>SMALEIHMSDPMCLIENFNEQLKVNQEALEILSAITQPVVVVAIVGLYRTGKSYLMNKLAGKNKGFSVASTVQSHTKGIWIWCVPHPNWPNHTLVLLDTEGLGDVEKADNKNDIQIFALALLLSSTFVYNTVNKIDQGAIDLLHNVTELTDLLKARNSPDLDRVEDPADSASFFPDLVWTLRDFCLGLEIDGQLVTPDEYLENSLRPKQGSDQRVQNFNLPRLCIQKFFPKKKCFIFDLPAHQK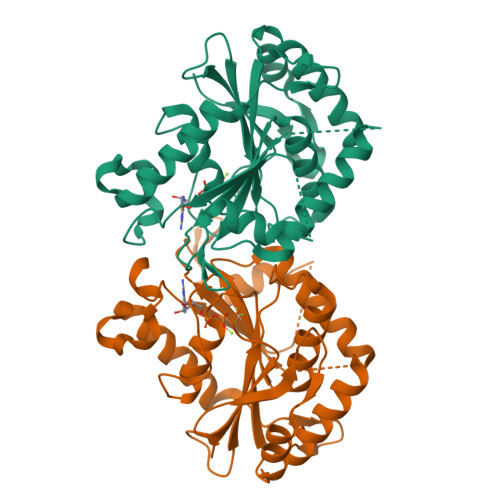KLAQLETLPDDELEPEFVQQVTEFCSYIFSHSMTKTLPGGIMVNGSRLKNLVLTYVNAISSGDLPCIENAVL[2x]> HHNKVRTCWNEGRPALAGWLQLPGTLHAEALARLDYDAVVIDMQHSPIDFGQVAPMLIAIELGGAEPFVRTQVNDPSD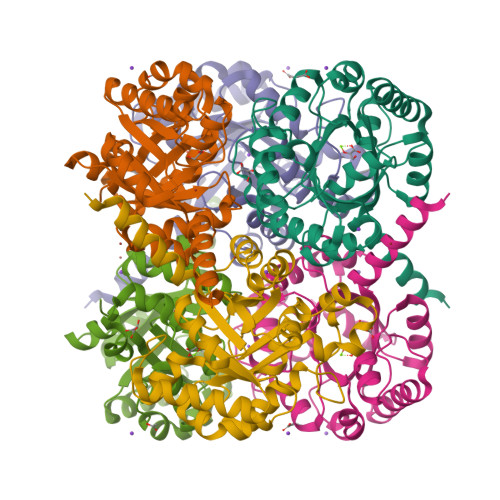IMKLLDAGAYGIIAPMVNTRAEAQTLASALHYSPRGLRSFGPRRPSLRYGSGYLAQASETVVGLAMIETREALANIDEILSVDGIDGVFIGPTDLALDLGHAPLVDTEEAEVVSAIAHVRERAHAAGKRVGIFCGSGGFARVKLAEGFDFVTAAPDLAMLSAAARQVIADARAL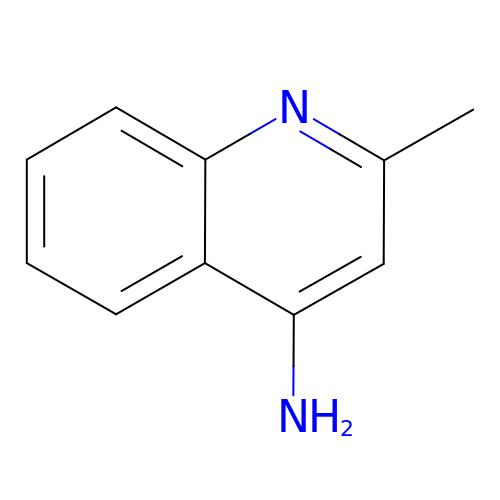2-methylquinolin-4-amine | C10 H10 N2 | COCFIBRMFPWUDW-UHFFFAOYSA-N>MNQNLLVTKRDGSTERINLDKIHRVLDWAAEGLHNVSISQVELRSHIQFYDGIKTSDIHETIIKAAADLISRDAPDYQYLAARLAIFHLRKKAYGQFEPPALYDHVVKMVEMGKYDNHLLEDYTEEEFKQMDTFIDHDRDMTFSYAAVKQLEGKYLVQNRVTGEIYESAQFLYILVAACLFSNYPRETRLQYVKRFYDAVSTFKISLPTPIMSGVRTPTRQFSSCVLIECGDSLDSINATSSAIVKYVSQRAGIGINAGRIRALGSPIRGGEAFHTGCIPFYKHFQTAVKSCSQGGVRGGAATLFYPMWHLEVESLLVLKNNRGVEGNRVRHMDYGVQINKLMYTRLLKGEDITLFSPSDVPGLYDAFFADQEEFERLYTKYEKDDSIRKQRVKAVELFSLMMQERASTGRIYIQNVDHCNTHSPFDPAIAPVRQSNLCLEIALPTKPLNDVNDENGEIALCTLSAFNLGAIN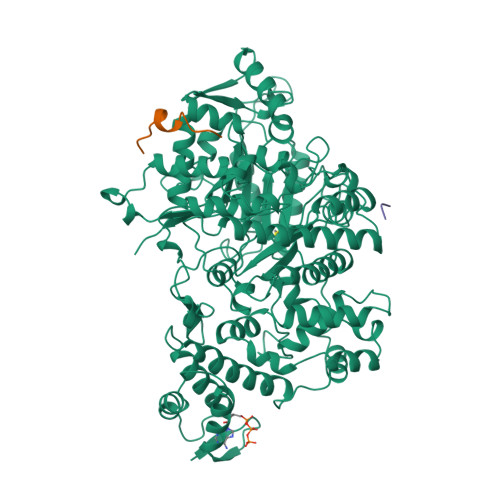NLDELEELAILAVRALDALLDYQDYPIPAAKRGAMGRRTLGIGVINFAYYLAKHGKRYSDGSANNLTHKTFEAIQYYLLKASNELAKEQGACPWFNETTYAKGILPIDTYKKDLDTIANEPLHYDWEALRESIKTHGLRNSTLSALMPSETSSQISNATNGIEPPRGYVSIKASKDGILRQVVPDYEHLHDAYELLWEMPGNDGYLQLVGIMQKFIDQSISANTNYDPSRFPSGKVPMQQLLKDLLTAYKFGVKTLYYQNTRDGAEDAQDDLVPSIQDDGCESGACKI[3x];>YLVGQIDSEVDTDDLSNFQL[4x]> HP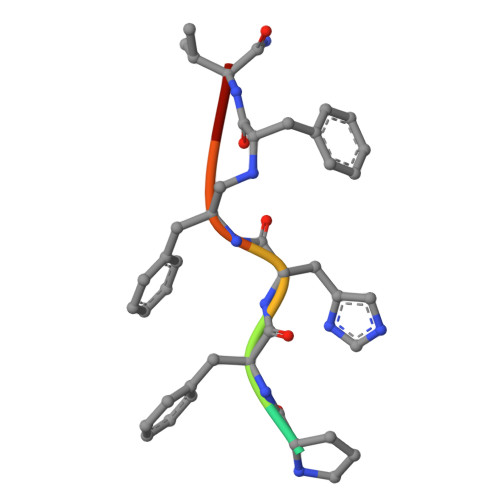FHXVY> GPLHMIDYKEIEVEEVVGRGAFGVVCKAKWRAKDVAIKQIESESERKAFIVELRQLSRVNHPNIVKLYGACLNPVCLVMEYAEGGSLYNVLHGAEPLPYYTAAHAMSWCLQCSQGVAYLHSMQPKALIHRDLKPPNLLLVAGGTVLKICDFGTACDIQTHMTNNKGSAAWMAPEVFEGSNYSEKCDVFSWGIILWEVITRRKPFDEIGGPAFRIMWAVHNGTRPPLIKNLPKPIESLMTRCWSKDPSQRPSMEEIVKIMTHLMRYFPGADEPLQYPCQHSLPPGEDGRVEPYVDFAEFYRLW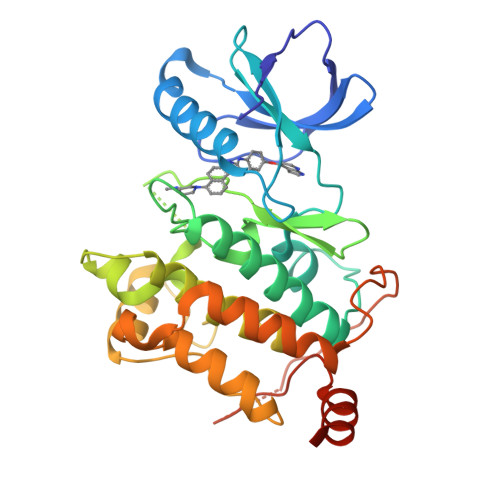SVDHGEQSVVTAP6-(m-tolylthio)-[1,2,4]triazolo[4,3-b]pyridazin-3(2H)-one | C12 H10 N4 O S | 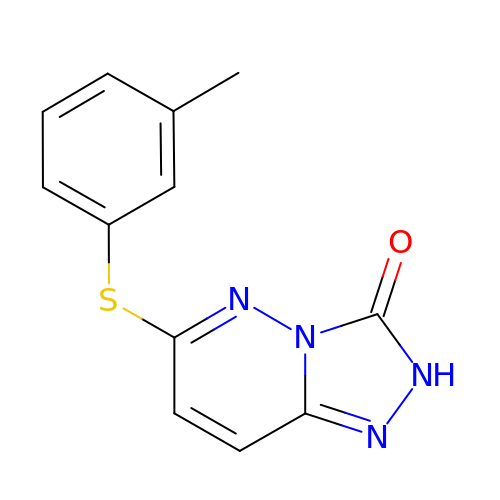VXFWYSKRDAZEEN-UHFFFAOYSA-N Cytochromes c′ (cyts c′) are a group of putative NO-binding heme proteins that fall into two families: the well-characterized four alpha helix bundle fold (cyts c′-α) and an unrelated family with a large beta-sheet fold (cyts c′-β) resembling that of cytochromes P460. Of these, cytochrome P460 (cytP460) is a heme enzyme that oxidizes hydroxylamine to N2O as part of nitrification (1), whereas the evolutionarily related cytochrome c′-β (cyt c′-β) binds the diatomic gases, NO and CO (2). By contrast, our recent crystal structure of cyt c′-β from Methylococcus capsulatus (Bath) (McCP-β) reveals a hydrophobic distal pocket dominated by two Phe residues (F32 and F61), a structural feature we have named the “Phe cap. Proposed roles for cyt c′-β proteins include protection against NO stress generated during nitrification.

We further probed the roles of the distal Phe cap residues (Phe 61 and Phe 32) by comparing the properties of wt McCP-β with those of the F32V and F61V variants, focusing on NO and CO complexes. Our goal in characterizing these aromatic → aliphatic variants was twofold: (i) to provide further evidence that the Phe 32 aromatic quadrupole limits Fe(II)→XO(π∗) backbonding and (ii) to establish the extent to which the Phe 32 aromatic quadrupole influences heme–gas reactivity. We assessed the impact of the Phe 32 aromatic quadrupole on McCP-β heme–gas affinity by comparing the structural, spectroscopic, and kinetic properties of wt McCP-β with those of the F61V and F32V variants.

>[2x]MNKPSFLLVGLLVVSGVLGAAETKVKYPDGFRSWYHVKSMVIQPGHPLENPFGGIHHVYANAEAIQGLRGGNYPDGAVLVVDLFDYQEDNHALVEGKRKLIGVMERDAKRFSATGGWGYEGFGEGKPDKRLVTDGGQGCFGCHAAQKESQYVFSRLRD>MTITLIEPVQQRTGIYPSSDLKVEDGYPSSDTFQIIQTQDGRGAGVRVLKTFARGRRMARVSGQITAFCRLHTLQINAHTHLYDPHFSGLLLHSCVPNVRLDMAGFELWSLRDIAAGEMLTMDYASTEDVLMRQFECHCGAPNCRRWITGAKELPNDIGQALLAGLRAAALALEHHHHHH[2x]

BurB, a SET (Suppressor of variegation, Enhancer of zeste and Trithorax) domain-containing enzyme identified from Burkholderia thailandensis, initiates DMSP synthesis by methylating methionine (Met) to S-methyl-methionine (SMM), with S-adenosyl methionine (SAM) as a methyl donor. BurB is a S-adenosyl methionine (SAM)-dependent Met S-methyltransferase containing a SET (Suppressor of variegation, Enhancer of zeste and Trithorax) domain, and belongs to the class V of the methyltransferase superfamilies. The SET domain proteins are well known for their roles in methylating histone lysines in eukaryotes, and BurB represents a new member of the SET domain proteins. Each BurB monomer consists of eight β-sheets and four α-helices.

The crystals of the BurB-Met complex belong to the C121 space group, with two BurB molecules arranged as a dimer in an asymmetric unit. The electron density map of the BurB-Met complex suggested that there is a Met molecule bound in the substrate binding site of BurB mainly by hydrogen bond interactions. Residues Arg70 and Thr73 can form hydrogen bonds with the nitrogen atom of Met. Met132 interacts with the carboxyl group of Met. Moreover, Val130 participates in Met binding by hydrogen bonds via a water molecule. It is noteworthy that all the residues interact with Met via their main chains, likely to enable a relatively stable Met’s binding pattern irrespective of potential mutations. In the BurB-Met complex, the Met molecule is accessible to the surface, suggesting that BurB possesses an open conformation. During catalysis, Met is firstly bound in the substrate binding pocket, while BurB maintains an open conformation for the subsequent binding of SAM. Thus, the binding of the Met molecule may occur before the binding of SAM in BurB, which is different from MmtN and DsyB.>MKEGFYWIQHNGRVQVAYYTHGVTEDL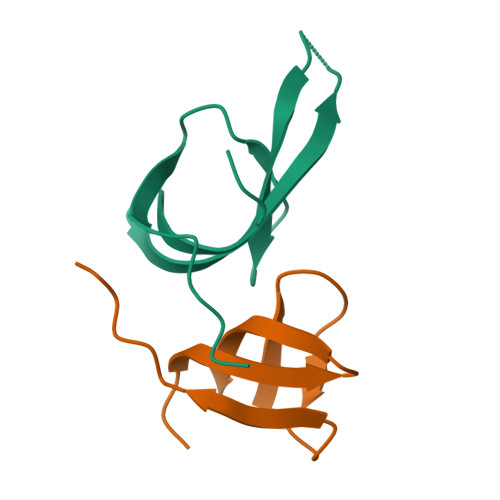ETGQTIIGVWHLTQGDDICHNGEAEILAGPLEPPI[2x]> MGDCDIEGKDGKQYESVLMVSIDQLLDSMKEIGSNCLNNEFNFFKRHICDANKEGMFLFRAARKLRQFLKMNSTGD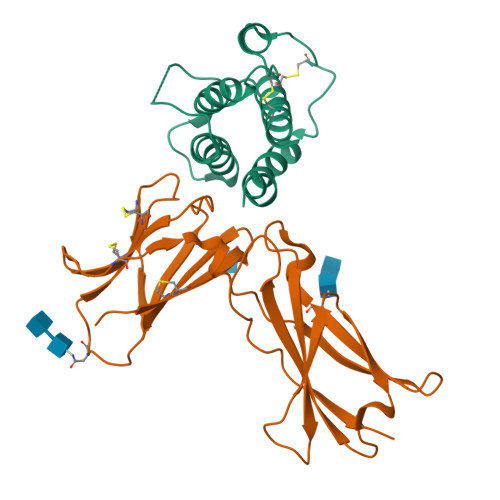FDLHLLKVSEGTTILLNCTGQVKGRKPAALGAAQPTKSLEENKSLKEQKKLNDLCFLKRLLQEIKTCWNKILMGTKEH;> GSHMESGYAQNGDLEDAELDDYSFSCYSQLEVNGSQHSLTCAFEDPDVNTTNLEFEICGALVEVKCLNFRKLQEIYFIETKKFLLIGKSNICVKVGEKSLTCKKIDLTTIVKPEAPFDLSVVYREGANDFVVTFNTSHLQKKYVKVLMHDVAYRQEKDENKWTHVNLSSTKLTLLQRKLQPAAMYEIKVRSIPDHYFKGFWSEWSPSYYFRTPEINNSSGEMD>MSNLLTVHQNLPALPVDATSDEVRKNLMDMFRDRQAFSEHTWKMLLSVCRSWAAWCKLNNRKWFPAEPEDVRDYLLYLQARGLAVKTIQQHLGQLNMLHRRSGLPRPSDSNAVSLVMRRIRKENVDAGERAKQALAFERTDFDQVRSLMENSDRCQDIRNLAFLGIAYNTLLRIAEIARIRVKDISRTDGGRMLIHIGR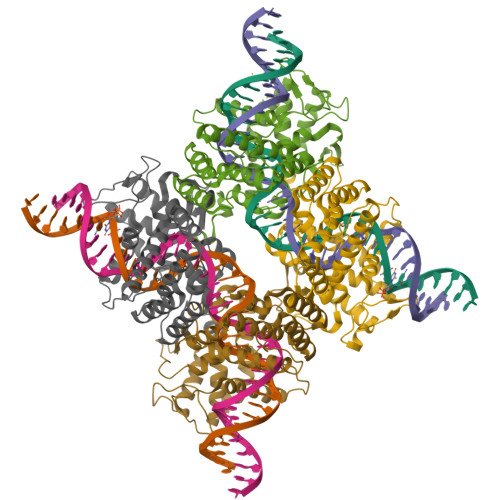TKTLVSTAGVEKALSLGVTKLVERWISVSGVADDPNNYLFCRVRKNGVAAPSATSQLSTRALEGIFEATHRLIYGAKDDSGQRYLAWSGHSARVGAARDMARAGVSIPEIMQAGGWTNVNIVMNYIRNLDSETGAMVRLLEDGD[4x]>MGRKKIQIQRITDERNRQVTFTKRKFGLMKKAYELSVLCDCEIALIIFNHSNKLFQYASTDMDKVLLKYTEYNEPHESRT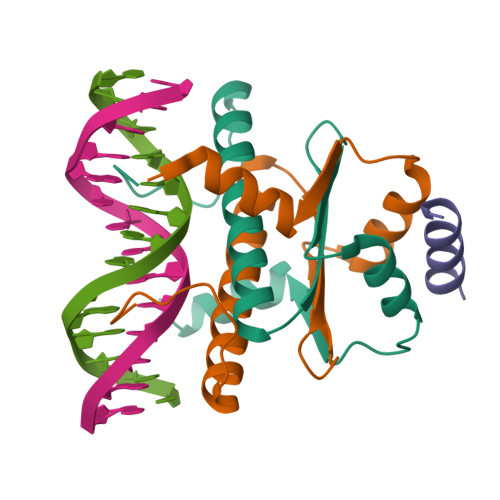NADIIETLRKKGFNG[4x];>GSGEVKMKLQEFVLNKK[2x]>GSQEKAVVLDEQAIRRALTRIAHEIIERNKGVDNCVLVGIKTRGIYLAKRLAERIEQIEGKKVPVGELDITLYRDDLTVTSNKEPLVKGTDIPVDITDKKVILVDDVLYTGRTVRAAMDALMDLGRPSQIQLAVLVDRGHRELPIRADYVGKNVPTSKSERIVVQLSEVDGQ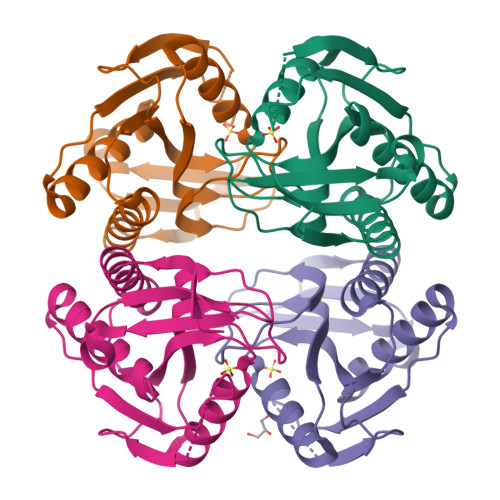DRVSIYEK[4x]>[3x]MVFHKKEPIHVVNIGEANPRFAQLLLEQFGGATGELSAALQYWVQSFHVENAGIKDML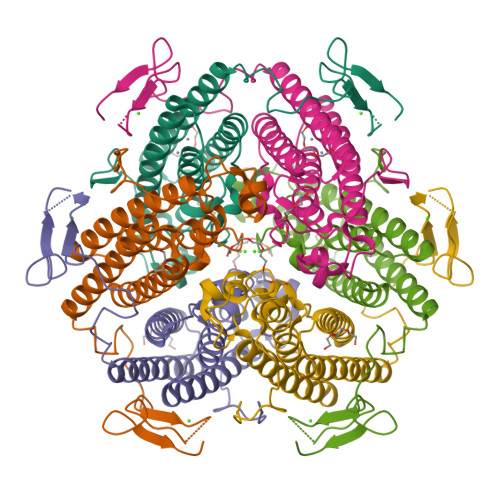QDIAIEEFSHLEMVGKLIEAHTKNVDQTEAYKSTLFAVRGMGPHFLDSQGNAWTASYLNEGGDVVRDLRANIAAEAGARQTYEELIKLSPDEGTKQTLVHLLTREISHTQMFMKALDSLGKLTDPFFGNVQPDETVALYYNLSSNGNGHDERGPWNSEPAFKYVANPLEKHSHHHHHH6-chloranyl-3-(2~{H}-indazol-5-yl)-~{N}-propan-2-yl-imidazo[1,2-b]pyridazin-8-amine | C16 H15 Cl N6 | 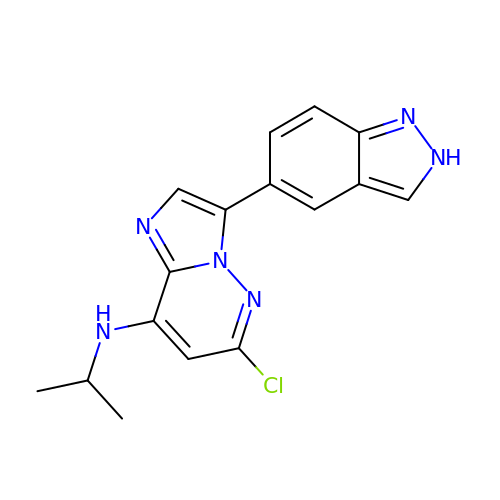TZFOHQPMYQZELA-UHFFFAOYSA-N4-[[(1E)-2-(4-CHLOROPHENYL)ETHENYL]SULFONYL]-1-[[1-(4-PYRIDINYL)-4-PIPERIDINYL]METHYL]PIPERAZINONE | C23 H27 Cl N4 O3 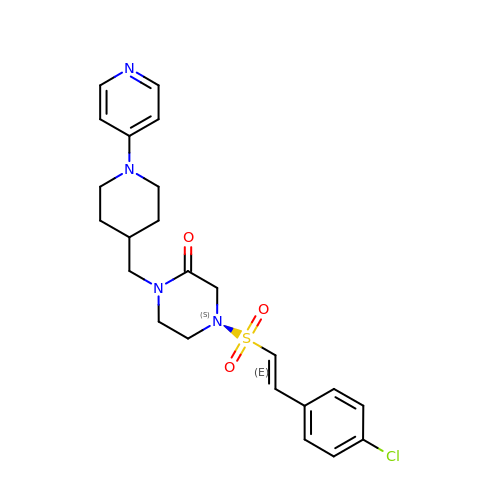S | QLHUDNKWOSQSMK-CXUHLZMHSA-N6-({4-[(4-cyanophenyl)amino]-1,3,5-triazin-2-yl}amino)-5,7- dimethyl-2-naphthonitrile | C23 H17 N7 | 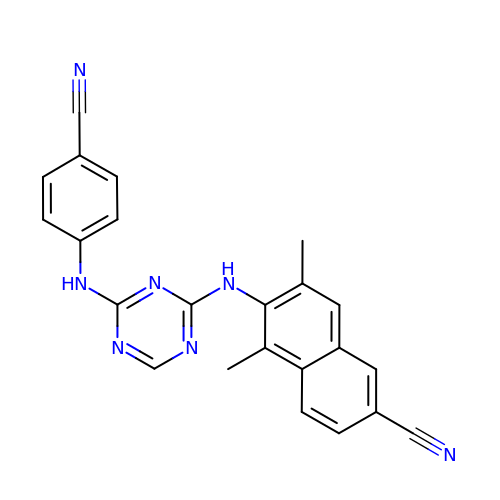KPKGAKOSWKZAAI-UHFFFAOYSA-N> TLFDNHPVQQYSGFNPIDFRFDDYVEGAKRFDNLA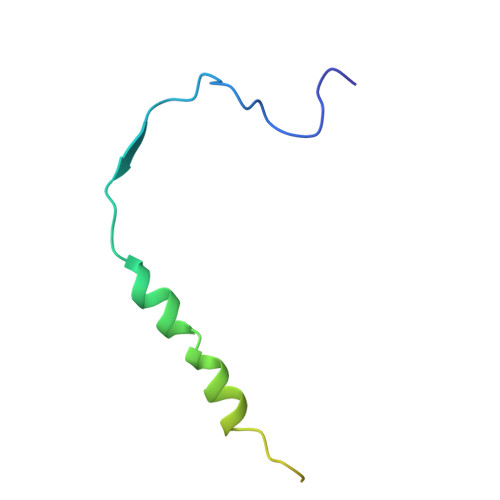NLIRSSTPTDPFANYQKPCESTSTSRSRTNSAKDQKHGP> EDDEDYGDLGGCPFLVAENKTGYPTIVACKQDCNGTTETAPNGTRCFSIGDEGLRRMTANLPYDCPLGQCSNGDCIPKETYEVCYRRNWRDKKNHH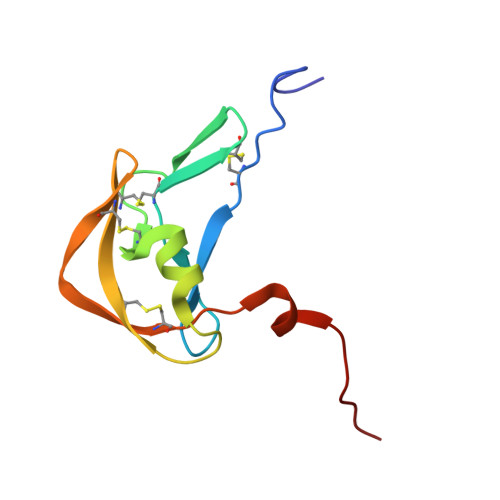HHHH>QHYFNSYDHYGIHEEMLQDTVRTLSYRNAIIQNKDLFKDKIVLDVGCGTGILSMFAAKHGAKHVIGVDMSSIIEMAKELVELNGFSDKITLLRGKLEDVHLPFPKVDIIISEWMGYFLLYESMMDTVLYARDHYLVEGGLIFPDKCSIHLAGLEDSQYKDEKLNYWQDVYGFDYS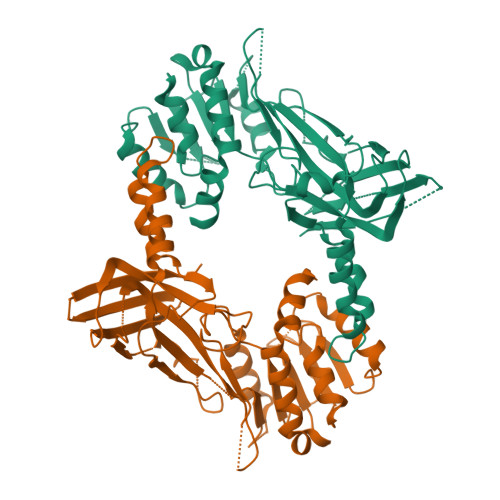PFVPLVLHEPIVDTVERNNVNTTSDKLIEFDLNTVKISDLAFKSNFKLTAKRQDMINGIVTWFDIVFPAPKGKRPVEFSTGPHAPYTHWKQTIFYFPDDLDAETGDTIEGELVCSPNEKNNRDLNIKISYKFESNGIDGNSRSRKNEGSYLMH[2x]DIUNDECYL PHOSPHATIDYL CHOLINE | 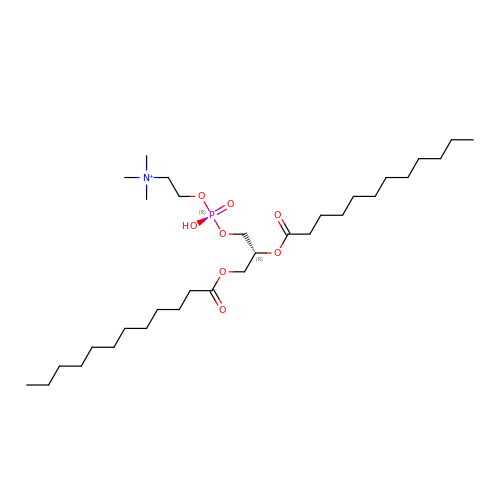C32 H65 N O8 P | IJFVSSZAOYLHEE-SSEXGKCCSA-O>[2x]MDFYYLPGSAPCRAVQMTAAAVGVELNLKLTDLMKGEHMKPEFLKLNPQHCIPTLVDNGFALWESRAI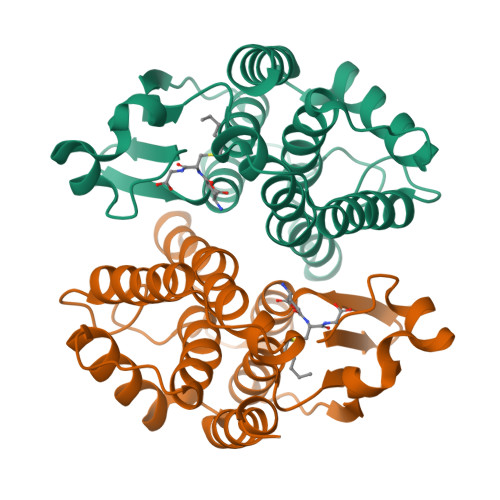QIYLAEKYGKDDKLYPKDPQKRAVVNQRLYFDMGTLYQRFADYHYPQIFAKQPANPENEKKMKDAVGFLNTFLEGQEYAAGNDLTIADLSLAATIATYEVAGFDFAPYPNVAAWFARCKANAPGYALNQAGADEFKAKFLS> 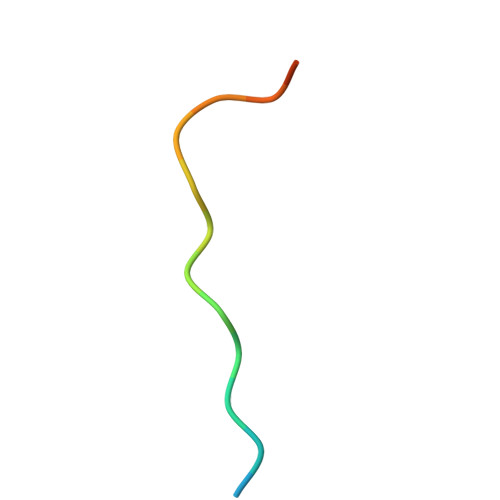XIGRRLPPTPSKPSTLX> SNNLII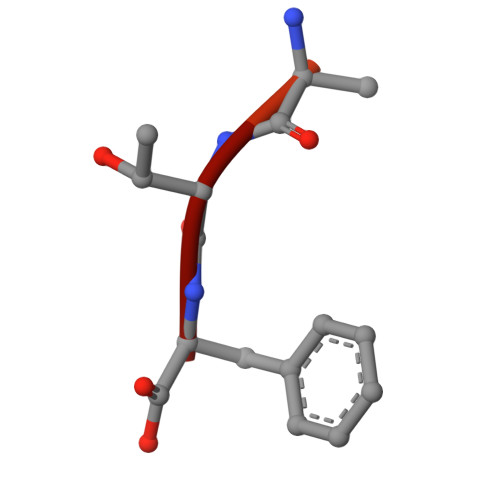DEETF> LPICPGGAARCQVTLRDLFDRAVVLSHYIHNLSSEMFSEFDKRYTHGRGFITKAINSCHTSSLATPEDKEQAQQMNQKDFLSLIVSILRSWNEPLYHLVTEVRG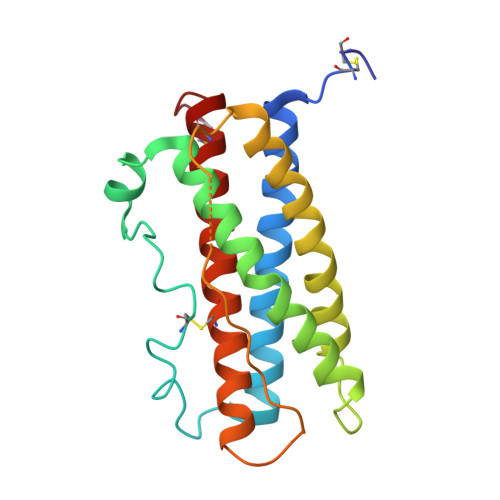MQEAPEAILSKAVEIEEQTKRLLEGMELIVSQVHPETKENEIYPVWSGLPSLQMADEESRLSAYYNLLHCLRRDSHKIDNYLKLLKCRIIHNNNC>[2x]SHKEFTKFCYEVYNEIKISDKEFKEKRAALDTLRLCLKRISPDAELVAFGSLESGLALKNSDMDLCVLMDSRVQSDTIALQFYEELIAEGFEGAFLQAARIPIIKLTSDTKNGFGASFQCDIGFNNRLAIHNTLLLSSYTKLDARLKPMVLLVKHWAKRKQINSPYFGTLSSYGYVLMVLYYLIHVIKPPVF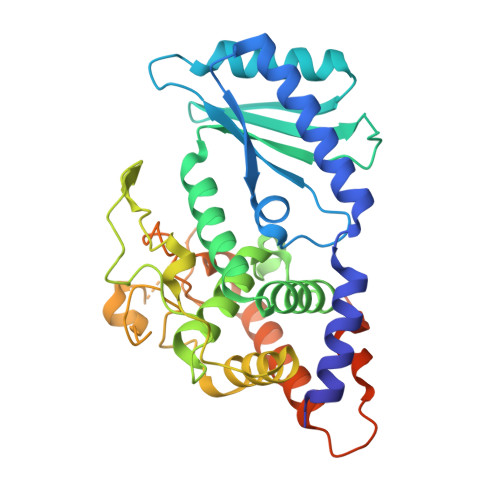PNLLLSPLKQEKIVDGFDVGFDDKLEDIPPSQNYSSLGSLLHGFFAFYAYAFEPREKVVTFRRPDGYLTKQEKGWTSATEHTGSADQIIKDRYILAIEDPFEISHNVGRTVSSSGLYRIRGEFMAASRLLNSRSYPIPYDSLFEEAPIPPRRQKKTDEQSNKKLLNETDGDNSE> MAPTQAGHDTAYLKETVGEALARGCAAAISAQPNDPVEYLGLWLLKYVKNAEVEGNFYRERQQDLQKKKDRLVKEAQSEQAAKSVALTRKEAADALALVTAEPRELLEAAVKLVKQHTAAGAAYAAVVAEPEEPDWVAPEDDEAAAVETEDEAAGGAALAEGEEPPPEPEPEPEAAPEDGEGDAPAPKIPRPVDYSKKYFAYVAASAGQEHVLEADLYRPAPPPEDADEDFKPEPLPYSFRVLDEKLPMLYVPNVAAEERVKFFRKFPKIGSYQACGVALPASGEFKALLAADTLFPEGSGQPLSADDRDFVWEVSQSLSRALEAVQARAAEALAATSAAEAVEELKAKVAELREQAAAEAAAAAPPPPAEGEEGEGEAPPAEEEPPAEEEAEEEEEEAEEGAEEGAEEGEEGEEAPPKPKKKKKVFNPIPGLQAAIEKLTAAAEAATEADARAQAAV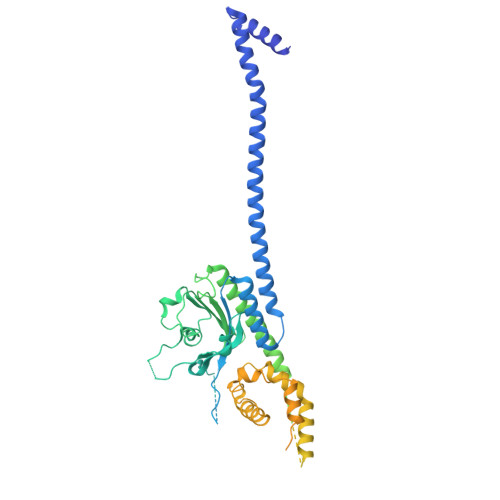ALEKQALDEVVALASSHSDATLSSLRNMLSVPQGTYHVVKALLHLLGRPAASFSTWKRAHSHFSPRLFEDMAAYDATAERDMAVWGRVRSCYKAAPAAKKLDAEMPNTLFGSVALMYIKQVRRVARKAVLQRELAAKLAKAQQDLADKQAALVEAERVKAEREAEEARLAAEAEAAAAAEAEAAARAAAEAEAAAAAEAAAEAAAEAAAAAAEAAAEAGEGEAVAEREAAPAEAEAAPAEGEAAPPAEGEGEAQPAQEGSNSSSSSSDSSSSEESKAAAE> FDVIGGNAYTIGGRSRCSIGFAVNGGFITAGHCGRTGATTANPTGTFAGSSFPGNDYAFVRTGAGVNLLAQVNNYSGGRVQV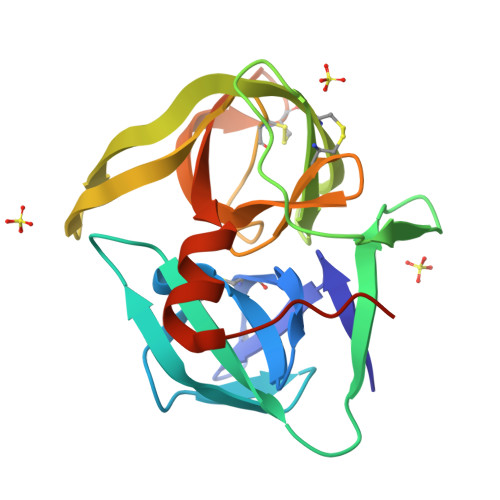AGHTAAPVGSAVCRSGSTTGWHCGTITALNSSVTYPEGTVRGLIRTTVCAEPGDSGGSLLAGNQAQGVTSGGSGNCRTGGTTFFQPVNPILQAYGLRMITTDSGSSP>[2x]SNAETIEIIKDLFEHLCGVRVHRTYEDDTGLWFDTSQGSKNGIMDYKLGFVKSQAENTTEVDTEVIYVPLLKQRTAEELQELQKKLPDYLFETLSFPLRSL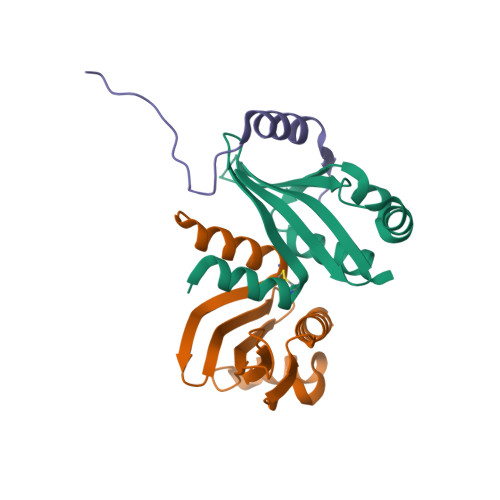NQFYIKMSKSLNKKV;> GDKDNGLHAGETDGDDEGFEFRRHSNLGVPTLGERLDSLHEIKSARRMDHFNSSRNSLR> VSRYVPDMGDLIWVDFDPTKGSEQAGHRPAVVLSPFMYNNKTGMCLCVPCTTQSKGYPFEVVLSGQERDGVALADQVKSIAWRARGATK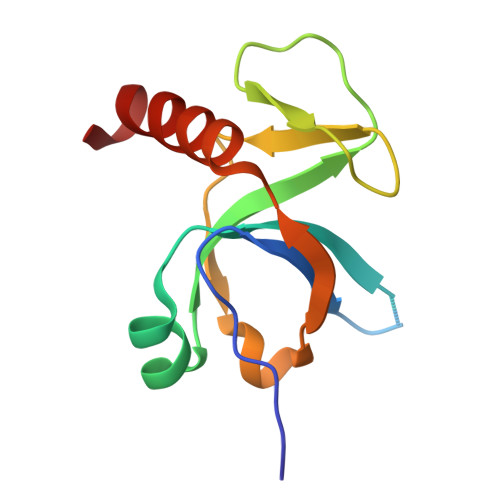KGTVAPEELQLIKAKINVLIG>[2x]MKKSELPDPFEKARESKGYGEMNDQDDPVTMLLRHKDVRKSAHNYKTFQSGAVPGRIVIPSEV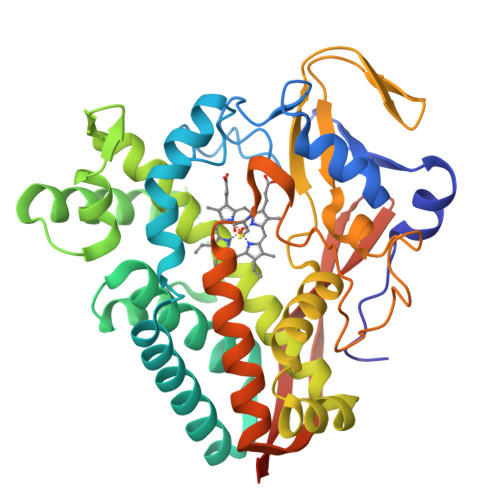DIRDTRQIPFEVDPPVHGVYRAIVEPWFKRPLQAEYQEKLTAQISEIVEETLLKGSVEVVTDFALRLQSRALTLLLNTPFSESETWISWGTHVFRSEGEALDGDKANILYHYIDEQIDRASENPGDDMYSVLLNSEFEGRKLTKEEVKGVMVLTFAGGRDTVINAVTNSIAYLAEHPEALERLRKEPEITGRAVEEMIRYFSPLTQMGRVVTEDTHVCEHAVKADSRISLCWASANRDAAVFENPNEIVLDRKVNPHVGFGFSHHNCLGATHARQILKILLQTLAQKVASFEILDYKENIEDLDHFQRKVGFHNIQIKFNPLTKLAAALEHHHHHH> MKLSPSMLDKLLRLGYSKLFADRYFQLWGERAIRIAEAMEKPLPRCFRVNTLKISVQDLVKRLNKKGFQFKRVPWAKEGFCLTREPFSITSTPEFLTGLIYIQEASSMYPPVALDPKPGEIVADMAAAPGGKTSYLAQLMRNDGVIYAFDVDENRLRETRLNLSRLGVLNVILFHSSSLHIGELNVEFDKILLDAPCTGSGTIHKNPERKWNRTMDDIKFCQGLQMRLLEKGLEVLKPGGILVYSTCSLEPEENEFVIQWALDNFDVELLPLKYGEPALTNPFGIELSEEIKNAR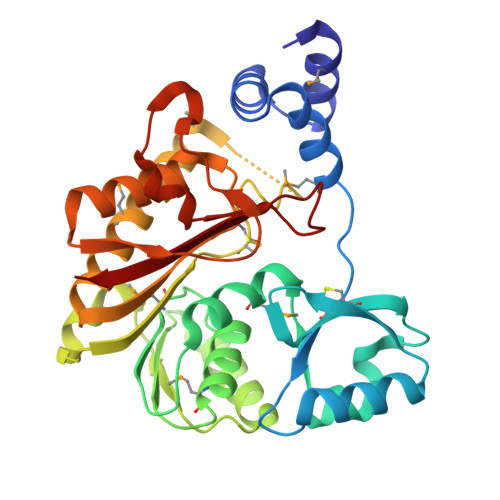RLYPDVHETSGFFIAKIRKL>AYTLATHTAGVIPAGKLERVDPTTVRQEGPWADPAQAVVQTGPNQYTVYVLAFAFGYQPNPIEVPQGAEIVFKITSPDVIHGFHVEGTNINVEVLPGEVSTVRYTFKRPGEYRIICNQYCGLGHQNMF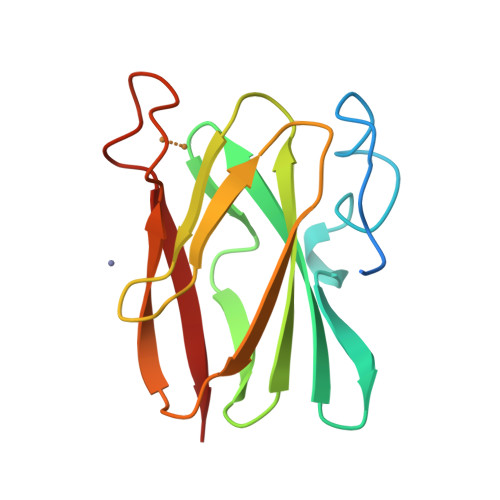GTIVVKE[2x]> SRSESSIESFFARGACV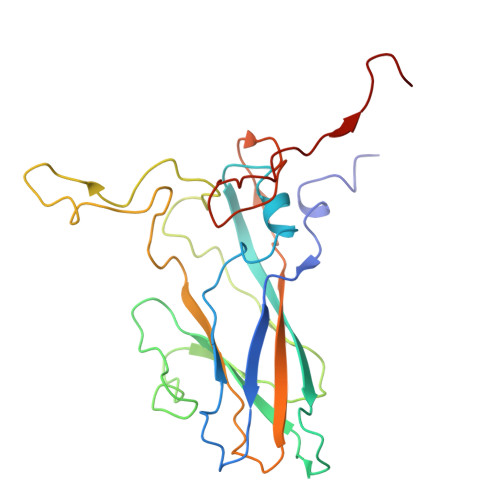TIMTVDNPASTTNKDKLFAVWKITYKDTVQLRRKLEFFTYSRFDMELTFVVTANFTETNNGHALNQVYQIMYVPPGAPVPEKWDDYTWQTSSNPSIFYTYGTAPARISVPYVGISNAYSHFYDGFSKVPLKDQSAALGDSLYGAASLNDFGILAVRVVNDHNPTKVTSKIRVYLKPKHIRVWCPRPPRAVAYYGPGVDYKDGTLTPLSTKDLTTY> WDIPTPKIIEECEYLEDGIYGIFQSTFLGASQRGVGVAQGGVFHTMWHVTRGAFLVRNGKKLVPSWASVKEDLVAYGGSWKLDGRWDGEEEVQLIAAAPGKNVVNVQTKPSLFKVKNGGEIGAVALDYPSGTSGSPIVNRNGEV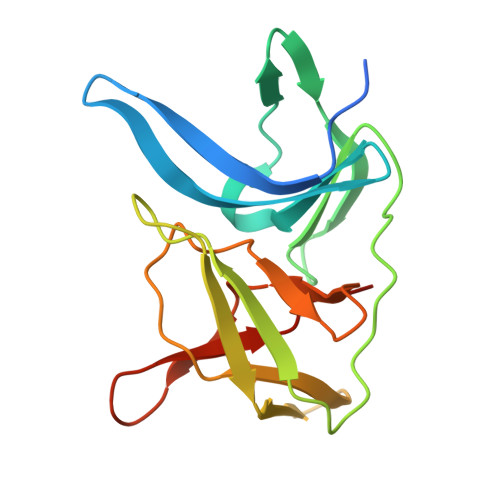IGLYGNGILVGDNSFVSAISQTEVKEE>MGSSHHHHHAMSEHRNEKGERISMINPRVVLDENGISHRSRYFIMLCDNETAIAHAKKTSIWAVKKDSSKRISDAYKKASVYFIFVAQQTYNALGYAQVVSDLNSTELPFWSDSSHAGGVRIKWIKTCNLFSAEISEIVSHMDHGSEARDGMEMMYDEGSRLCTLINYAIM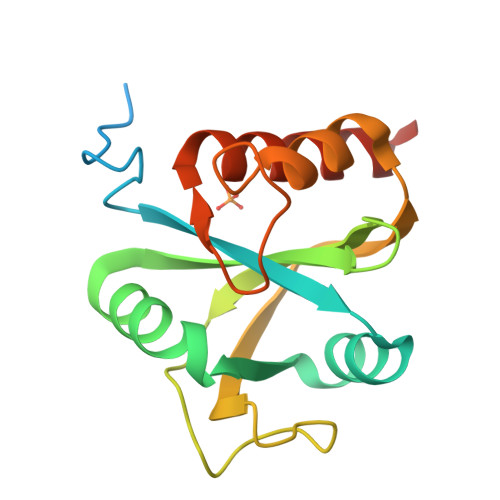KRIGRDR[2x]>[2x]VPDSIDYRKKGYVTPVKNQGQCGSCWAFSSAGALEGQLKKKTGKLLALSPQNLVDCVTENYGCGGGY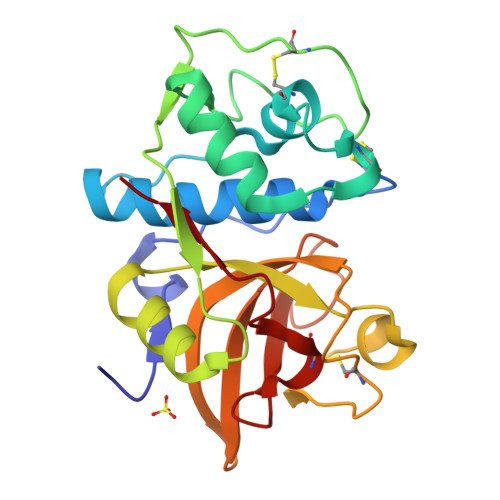MTTAFQYVQQNGGIDSEDAYPYVGQDESCMYNAAAKAAKCRGYREIPVGNEKALKRAVARVGPISVSIDASLASFQFYSRGVYYDENCDRDNVNHAVLVVGYGTQKGSKHWIIKNSWGESWGNKGYALLARNKNNACGITNMASFPKM>[2x]GSHMTNIPGLKKLWSETRGDPKICVAVLDGIVDQNHPCFIGADLTRLPSLVSGEANANGSMSTHG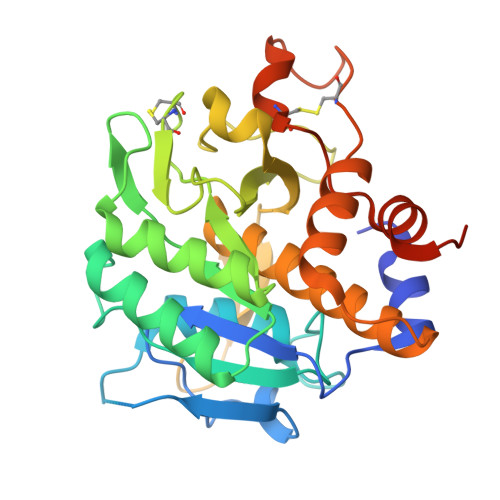THVASIIFGQHDSPVTGIAPQCRGLIVPVFADESLKLSQLDLSRAIEQAVNNGANIINVSAGQLTDAGEADTWLEKAIQLCQENNVLLIAATGNDGCECLHVPASLPTVLAVGAMDDQGKPVDFSNWGDAYQKQGILAPGKDILGAKPNGGTIRLSGTSFATPIVSGVAALLLSLQIKRGEKPDPQKVKNALLASATPCNPKDTDDQSRCLMGKLNILDAIEHLTGETMSEDLELESVEAS>MAAKQQERTYIMVKPDGVQRGLVSEVIRRFEQRGYKLVALKMKSPDATLLEEHYADLKGKPFFPGLISYMTSGPVVCMVWEGTDVVKQGRRMLGETRPLESNPGTLRGDFCIDVGRNIVHGSDSVESANKEISLWFTPEEICEWTSAQHKWVYEQGENLYFQSAGHHHHHH[12x]

Toxoplasma gondii is one of the most significant parasites that impacts human health, with estimates that as many as one third to one half of the human population are infected. At the Center for Structural Genomics of Infectious Diseases (CSGID), the first Toxoplasma Structural Genomics Pipeline was established. The enzymes selected from the TDR database as small and tractable for expression and crystallization included: phosphoglycerate mutase II (hereafter referred to as PGM), nucleotide diphosphate kinase (NDK), ribulose phosphate 3-epimerase (RPE), ribose-5-phosphate isomerase (RPI), and ornithine aminotransferase (OAT). The genes encoding these enzymes were cloned, proteins expressed and purified, crystallized, and crystal structures were determined.

Nucleotide diphosphate kinase catalyzes the movement of phosphate from a nucleoside triphosphate to a nucleoside diphosphate (e.g., GTP + ADP –> GDP + ATP). In both structures, TgNDK forms a hexamer with an average BSA of ~18,900 Å2. Comparison of TgNDK with known crystal structures of homologs proteins suggests that the TgNDK hexamer is likely a biologically functional assembly. TgNDK adopts an α/β/α sandwich fold with four β strands and eight surrounding α helices. Crystal structure of TgNDK suggests that the protein forms a hexamer with conserved nucleotide binding sites. Pairwise structural alignment revealed that active site of TgNDK may undergo similar conformational changes as its closest homolog, humanNM23-H2 transcription factor. On the other hand, when the dinucleotide is absent, the active site loop comprising of residues G59-F62 (Tg numbering) is shifted significantly (3–4 Å) between species. Additionally, TgNDK residue K60 is residue R58 in the human ortholog, offering different hydrogen-bond capacities to putative ligands. These observations suggest opportunities for the selective design of TgNDK inhibitors using structure-based molecular modeling techniques. TgNDK (+2.45) also appeared to be dispensable in tachyzoites.>MPIRVPDELPAVNFLREENVFVMTTSRASGQEIRPLKVLILNLMPKKIETENQFLRLLSNSPLQVDIQLLRIDSRESRNTPAEHLNNFYCNFEDIQDQNFDGLIVTGAPLGLVEFNDVAYWPQIKQVLEWSKDHVTSTLFVCWAVQAALNILYGIPKQTRTEKLSGVYEHHILH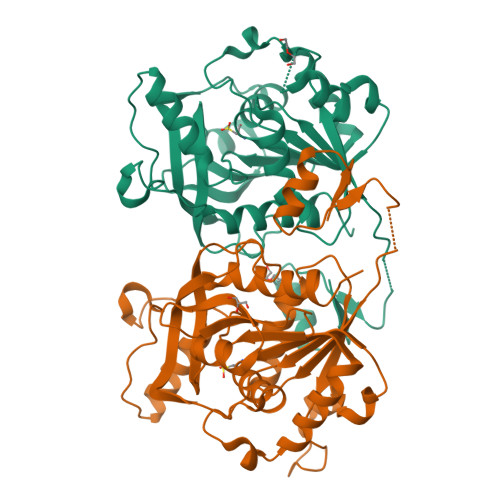PHALLTRGFDDSFLAPHSRYADFPAALIRDYTDLEILAETEEGDAYLFASKDKRIAFVTGHPEYDAQTLAQEFFRDVEAGLDIDVPYNYFPHNDPQNTPRASWRSHGNLLFTNWLNYYVYQIHHHHHH[2x]>PISKMVTAHFVLIHTICHGAWIWHKLKPALERAGHKVTALDMAASGIDPRQIEQINSFDEYSEPLLTFLEKLPQGEKVIIVGESCAGLNIAIAADRYVDKIAAGVFHNSLLPDTVHSPSYTVEKLLESFPDWRDTEYFTFTNITGETITTMKLGFVLLRENLFTKCTDGEYELAKMVMRKGSLFQNVLAQRPKFTEKGYGSIKKVYIWTDQDKIFLPDFQRWQIANYKPDKVYQVQGGDHKLQLTKTE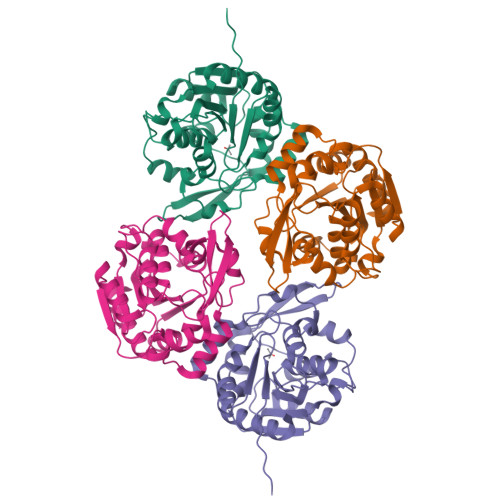EVAHILQEVADAYA[2x]> MDPYCPFDALDVWEHRRFIVADSRNFITPEFPRDFWMSPVFNLPRETAAEQVVVLQAQRTAAAAALENAAMQAAELPVDIERRLRPIERNVHEIAGALEALETAAAAAEEADAARGDEPAGGGDGGAPPGLAVAEMEVQIVRNDPPLRYDTNLPVDLLHMVYAGRGATGSSGVVFGTWYRTIQDRTITDFPLTTRSADFRDGRMSKTFMTALVLSLQSCGRLYVGQRHYSAFECAVLCLYLLYRNTHGAADDSDRAPVTFGDLLGRLPRYLACLAAVIGTEGGRPQYRYRDDKLPKTQFAAGGGRYEHGALASHIVIATLMHHGVLPAAPGDVPRDASTHVNPDGVAHHDDINRAAAAFLSRGHNLFLWEDQTLLRATANTITALGVIQRLLANGNVYADRLNNRLQLGMLIPGAVPSEAIARGASGSDSGAIKSGDNNLEALCANYVLPLYRADPAVELTQLFPGLAALCLDAQAGRPVGSTRRVVDMSSGARQAALVRLTALELINRTRTNPTPVGEVIHAHDALAIQYEQGLGLLAQQARIGLGSNTKRFSAFNVSSDYDMLYF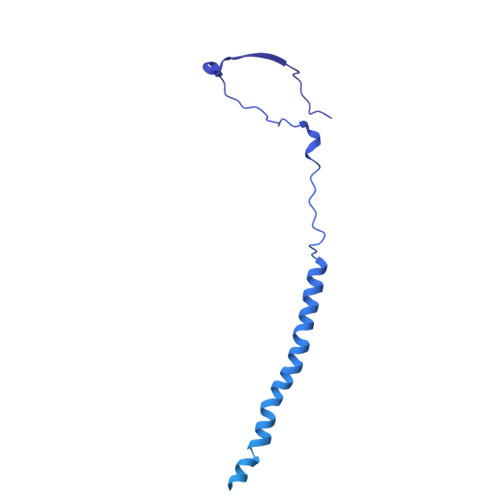LCLGFIPQYLSAV>[2x]IVGGYTCQENSVPYQVSLNSGYHFCGGSLINDQWVVSAAHCYKSRIQVRLGEHNINVLEGNEQFVNAAK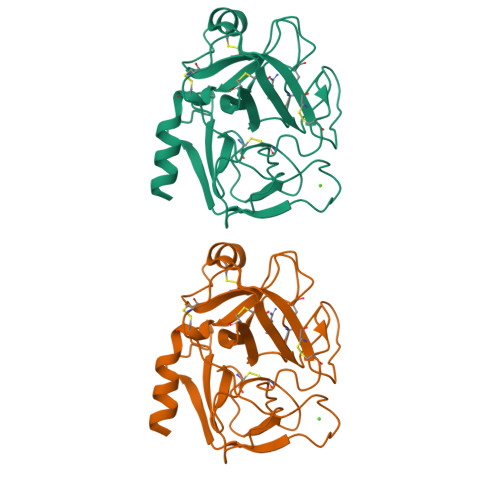IIKHPNFDRKTLNNNIMLIKLSSPVKLNARVATVALPSSCAPAGTQCLISGWGNTLSSGVNEPDLLQCLDAPLLPQADCEASYPGKITDNMVCVGFLEGGKDSCQGDSGGPVVCNGELQGIVSWGYGCALPDNPGVYTKVCNYVDWIQDTIAAN>[4x]M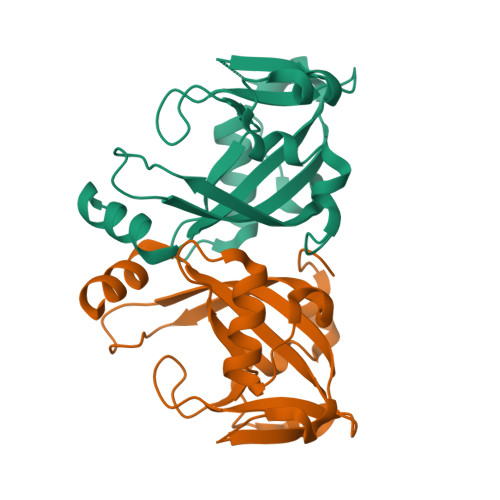MFLRQEDFATVVRSTPLVSLDFIVENSRGEFLLGKRTNRPAQGYWFVPGGRVQKDETLEAAFERLTMAELGLRLPITAGQFYGVWQHFYDDNFSGTDFTTHYVVLGFRFRVSEEELLLPDEQHDDYRWLTSDALLASDNVHANSRAYFLAEKRTGVPGL> MSAVALPRVSGGHDEHGHLEEFRTDPIGLMQRVRDELGDVGTFQLAGKQVVLLSGSHANEFFFRAGDDDLDQAKAYPFMTPIFGEGVVFDASPERRKEMLHNAALRGEQMKGHAATIEDQVRRMIADWGEAGEIDLLDFFAELTIYTSSATLIGKKFRDQLDG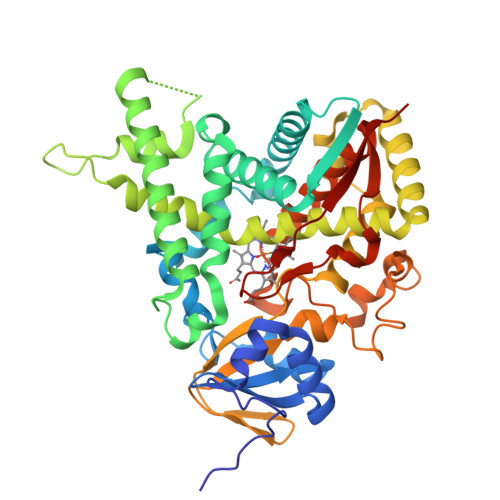RFAKLYHELERGTDPLAYVDPYLPIESFRRRDEARNGLVALVADIMNGRIANPPTDKSDRDMLDVLIAVKAETGTPRFSADEITGMFISMMFAGHHTSSGTASWTLIELMRHRDAYAAVIDELDELYGDGRSVSFHALRQIPQLENVLKETLRLHPPLIILMRVAKGEFEVQGHRIHEGDLVAASPAISNRIPEDFPDPHDFVPARYEQPRQEDLLNRWTWIPFGAGRHRCVGAAFAIMQIKAIFSVLLREYEFEMAQPPESYRNDHSKMVVQLAQPAAVRYRRRTGVHHHH> MGSSHHHHHHQNVSLQPPPQQLIVQNKTIDLPAVYQLNGGEEANPHAVKVLKELLSGKQSSKKGMLISIGEKGDKSVRKYSRQIPDHKEGYYLSVNEKEIVLAGNDERGTYYALQTFAQLLKDGKLPEVEIKDYPSVRYRGVVEGFYGTPWSHQARLSQLKFYGKNKMNTYIYGPKDDPYHSAPNWRLPYPDKEAAQLQELVAVANENEVDFVWAIHPGQDIKWNKEDRDLLLAKFEKMYQLGVRSFAVFFDDISGEGTNPQKQAELLNYIDEKFAQVKPDINQLVMCPTEYNKSWSNPNGNYLTTLGDKLNPSIQIMWTGDRVISDITRDGISWINERIKRPAYIWWNFPVSDYVRDHLLLGPVYGNDTTIAKEMSGFVTNPMEHAESSKIAIYSVASYAWNPAKYDTWQTWKDAIRTILPSAAEELECFAMHNSDLGPNGHGYRREESMDIQPAAERFLKAFKEGKNYDKADFETLQYTFERMKESADILLMNTENKPLIVEITPWVHQFKLTAEMGEEVLKMVEGRNESYFLRKYNHVKALQQQMFYIDQTSNQNPYQPGVKTATRVIKPLIDRTFATVVKFFNQKFNAHLDATTDYMPHKMISNVEQIKNLPLQVKANRVLISPANEVVKWAAGNSVEIELDAIYPGENIQINFGKDAPCTWGRLEISTDGKEWKTVDLKQKESRLSAGLQKAPVKFVRFTNVSDEEQQVYLRQFVLTIEKK;> MGSSHHHHHHQQVSLQPPPQQLIVQNKTIDLPAVYQLNGGEEANPHAVKVLKELLSGKQSSKKGMLISIGEKGDKSVRKYSRQIPDHKEGYYLSVNEKEIVLAGNDERGTYYALQTFAQLLKDGKLPEVEIKDYPSVRYRGVVEGFYGTPWSHQARLSQLKFYGKNKMNTYIYGPKDDPYHSAPNWRLPYPDKEAAQLQELVAVANENEVDFVWAIHPGQDIKWNKEDRDLLLAKFEKMYQLGVRSFAVFFDDISGEGTNPQKQAELLNYIDEKFAQVKPDINQLVMCPTEYNKSWSNPNGNYLTTLGDKLNPSIQIMWTGDRVISDITRDGISWINERIKRPAYIWWNFPVSDYVRDHLLLGPVYGNDTTIAKEMSGFVTNPMEHAESSKIAIYSVASYAWNPAKYDTWQTWKDAIRTILPSAAEELECFAMHNSDLGPNGHGYRREESMDIQPAAERFLKAFKEGKNYDKADFETLQYTFERMKESADILLMNTENKPLIVEITPWVHQFKLTAEMGEEVLKMVEGRNESYFLRKYNHVKALQQQMFYIDQTSNQNPYQPGVKTATRVIKPLIDRTFATVVKFFNQKFNAHLDATTDYMPHKMISNVEQIKNLPL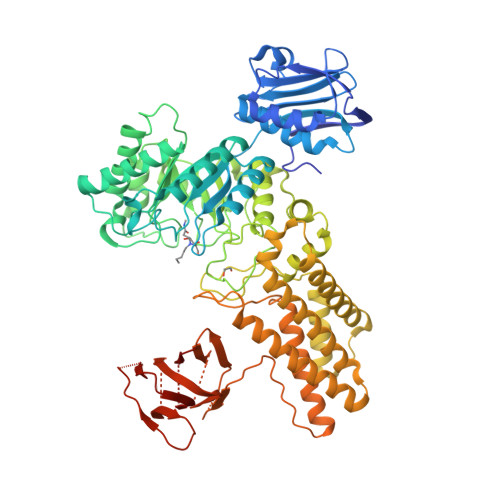QVKANRVLISPANEVVKWAAGNSVEIELDAIYPGENIQINFGKDAPCTWGRLEISTDGKEWKTVDLKQKESRLSAGLQKAPVKFVRFTNVSDEEQQVYLRQFVLTIEKK>GPLGSSAPSVKGVSFDQANNLLIEPARIEEEELTLTILRQTGGLGISIAGGKGSTPYKGDDEGIFIS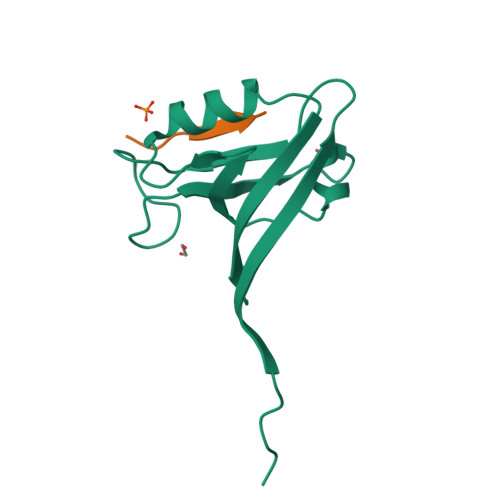RVSEEGPAARAGVRVGDKLLEVNGVALQGAEHHEAVEALRGAGTAVQMRVWRERM[2x];>LQSETSV[2x]>[3x]TNEVEECENYFSKTLLDRKSEKRNNSDWLLAKESHPATVFILFSDLNPLVTLGGNKESFQQPEVRLCQLNYTDIKDYLAQPEKITLIFLGVELEIKDKLLNYAGEVPREEEDGLVAWFALGIDPIAAEEFKQRHENCYFLHPPMPALLQLKEKEAGVVAQARSVLAWHSRYKFCPTCGNATKIEEGGYKRLCLKEDCPSLNGVHN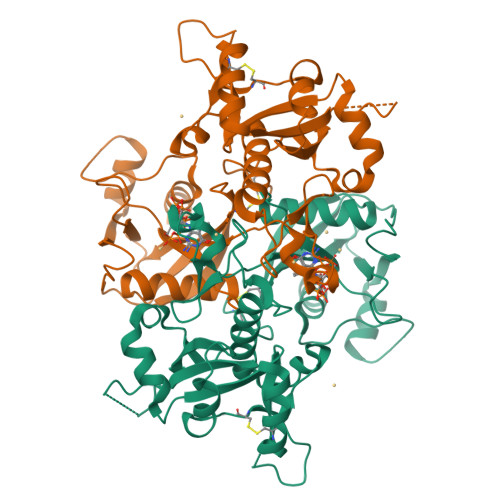TSYPRVDPVVIMQVIHPDGTKCLLGRQKRFPPGMFTCLAGFIEPGETIEDAVRREVEEESGVKVGHVQYVACQPWPMPSSLMIGCLALAVSTEIKVDKNEIEDARWFTREQVLDVLTKGKQQAFFVPPSRAIAHQLIKHWIRINPNL>[4x]DGENLRPVVINGSNVAMSHGNKEVFSCRGIKLAVDWFLER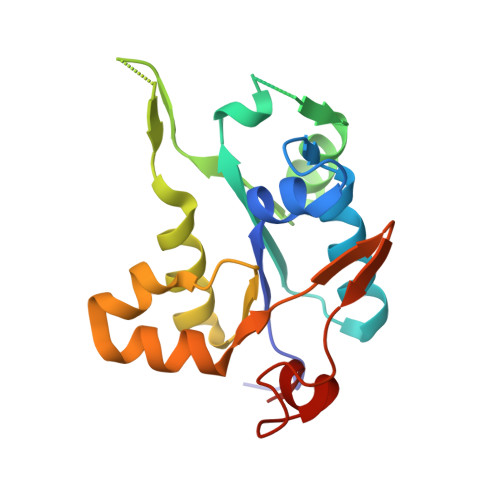GHKDITVFVPAWRKEQSRPDALITDQEILRKLEKEKILVFTPSRRVQGRRVVCYDDRFIVKLAFESDGIIVSNDNYRDLANEKPEWKKFIDERLLMYSFVNDKFMPPDDPLGRHGPSLDNFLRK> MKKIILGLSVLCLLMACGSSEQPAVIKVSEETLMYEVRATPSPADGTYVKVNPPRFMWPDKFPHLGPVLDGVPGQVDEKPKVVYRIRISQDKNFRKDVLTGERAWAFFNPFQCLAQGKWYWQHAYVTPEGTEEWSPVYQFYIDKDTPEFNPPTLEKVLARYPSHHPRVLLDADDWENIIAKNNNNPEARTYMDKASQCISRPLKHLQEEIDTTNVVTLTNIVQRESALIRESRKIVDREEANVEALVRAYLLTKDEKYYREGINRLSEILSWQKSKYFAGDFNLSTLLSMSTSAYDGFYNLLSPEEKQLLLDNIRKIGDKFYNEYVNHLENRIADNHVWQMTFRILTMAAFATVGEIPEASVWTDYCYNEWISRLPGLHKDGGWHNGDAYFHVNIRTLIEVPVFFSRISGFNFFADPWYNNNALYVIYQQPPFSKSGGHGNSHEGQRSPNGGRIGYADALARECNNPWAAAYVHEIMQEDPDILSKAFEAKPADLTWYRCTTPKERPAYSKHLSELPESKVFKQTGTALMNTDIGHHANNAMLSFRSSPYGSTSHALANQNAFNTFFGGKAIFYSSGHRTGFTDDHCMYAYRNTRAHNSILVNGMGQKIGTEGYGWIPRYYEGEEISYVVGDASNAYGKVVSPLWLERGRLSGTQFTPEKGWDENKLEFFRRHVVQLGRSGLFVVYDELAGKEPVEWNYLLHTVELPMEVVKEEGGLRILGKNKADGISIAHLYSSQEMTYAQTDTFFVAALDWKKRLGKALPNHYHFTATTAPCNKVFFLNIIDVHGNNRADAVINHQGNHITVEGWVIECNLDSEGKAFLHIENKQNGASLDFNYNSNKGATTIVDQVDGKRIEKRLVDSLPEPEILEHHHHHH

Herein, a type of exolytic heparinases (exoHepases) is identified from the genomes of different bacteria. These exoHepases share almost no homology with known Hepases and prefer to digest HP rather than HS chains by sequentially releasing unsaturated disaccharides from their reducing ends. The structure of BIexoHep consists of three domains: an N-terminal small β-sheet domain (Ala24–Asn150) composed of a large loop and a five-stranded β-sheet (β1–β5), a central (α/α)5 barrel domain (Pro151–Glu515) containing 20 α-helices (α1–α20) to form an (α/α)5 incomplete toroid structure, and a C-terminal β-sandwich domain (Leu516–Pro864) containing 23 β-strands and 5 short α-helices that fold into a three-layered β-sheet sandwich structure (α21–α25 and β6–β28). Further structural studies have shown that the active center of the exolytic Hepase is an L-shaped semiopen tunnel with a positively charged entrance and a negatively charged exit, which precisely controls the sequential cleavage of highly negatively charged HP.

To investigate the structural characteristics of the PL15_2 proteins, the crystal structure of BIexoHep with an HP disaccharide product was solved at a resolution of 1.98 Å by preparing a crystal of selenomethionine (SeMet)-labeled BIexoHep in the presence of HP disaccharide products followed by single-wavelength anomalous dispersion (SAD) phasing. In the crystal structures, each asymmetric unit consists of one BIexoHep monomer, an unsaturated disaccharide (ΔUA2S1-4GlcNS6S) or tetrasaccharide (ΔUA1-4GlcNS6S1-4IdoA2S1-4GlcNS6S), and two Ca2+ ions that were confirmed by inductively coupled plasma-mass spectrometry (ICP-MS) analysis. Notably, the BIexoHep complex with the disaccharide product and the structure with the tetrasaccharide substrate do not show significant differences (the root-mean-square deviation (r.m.s.d.) between the two structures was 0.140 Å based on 786 atoms). According to the hydrogen-bonding networks, a series of residues, such as Asp70, Ser226, Arg230, Arg233, Arg332, Asn336, His337, Gln340, Tyr390, Ser554, His555, Arg579, Arg648, Lys755, and Arg757, participate in the binding of the disaccharide product (ΔUA2S1-4GlcNS6S) and the tetrasaccharide substrate (ΔUA1-4GlcNS6S1-4IdoA2S1-4GlcNS6S). The negatively charged residues Pro67, Asp70, Pro73, Asp281, Glu234, and Asp335 from the N-terminal small β-sheet and central (α/α)5 barrel domains compose the negatively charged section of the tunnel for quick delivery of the disaccharide product. The mutation of negatively charged Asp residues to uncharged Ala or Asn or positively charged His in the exit tunnel caused a dramatic decrease of enzyme activity, such as the enzyme activities of mutants BIexoHep-P67A, BIexoHep-D70N, BIexoHep-D281A, BIexoHep-D281N and BIexoHep-D281H are reduced by 90%, 98%, 70%, 68%, and 85%, respectively, compared with that of the WT-BIexoHep.> ILPQPDVRVNQVGYLPEGKKVATVVCNSTQPVKWQLKNAAGVVVLEGYTEPKGLDKDSQDYVHWLDFSDFATEGIGYYFELPTVNSPTNYSHPFDIRKDIYTQMKYDALAFFYHKRSGIPIEMPYAGGEQ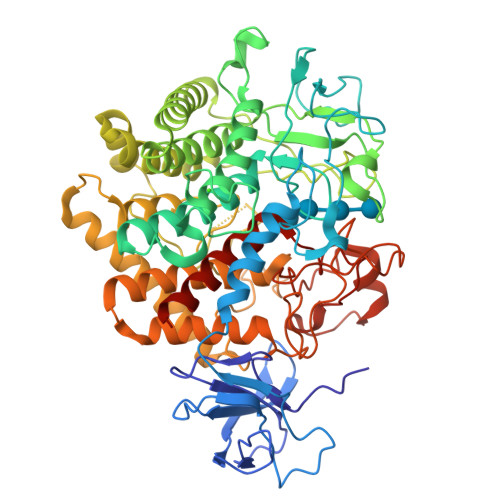WTRPAGHIGIEPNKGDTNVPTWPQDDEYAGIPQKNYTKDVTGGWYDAGDHGKYVVNGGIAVWTLMNMYERAKIRGLDNWGPYRDGGMNIPEQNNGYPDILDEARWEIEFFKKMQVTEKEDPSIAGMVHHKIHDFRWTALGMLPHEDPQPRYLRPVSTAATLNFAATLAQSARLWKDYDPTFAADCLEKAEIAWQAALKHPDIYAEYTPGSGGPGGGPYNDDYVGDEFYWAACELYVTTGKDEYKNYLMNSPHYLEMPAKMGENGGANGEDNGLWGCFTWGTTQGLGTITLALVENGLPATDIQKARNNIAKAADRWLENIEEQGYRLPIKQAEDERGGYPWGSNSFILNQMIVMGYAYDFTGDSKYLDGMFDGISYLLGRNAMDQSYVTGYGERPLQNPHDRFWTPQTSKRFPAPPPGIISGGPNSRFEDPTINAAVKKDTPPQKCFIDHTDSWGTNQITVNWNAPFAWVTAYLDEQYTD>[3x]MSASPPISAGDYLSAPEPDALKPAGPTPSQSRFQVDLVTESAGDGETTVGFDSSPPEYVAEPPPDGLRDSVSGGEKAKGRFRVVNFAASSPDAAPAETAQNGDTVMSEGSLHSSTGGQQHHHYDTHTNTYYLRTFGHNTIDAVPKIDFYRQTAAPLGEKLIRPTLSELHDELDKEPFEDGFANGEELTPAEESAAKDVSESKEPVRFGWVKGVMIRCMLNIWGVILYLRLPWITAQAGIVLTWIIILLSVTVTSITGLSISAISTNGKVKSGGTYFLISRSLGPELGGSIGLIFAFANAVGVAMHTVGFAATVRDLLQEYGAPIVDPINDIRIIGVVSVTVLLAISLAGMEWESKAQVLFFLVIMVSFANYLVGTLIPPSEDKASKGFFSYRADIFVQNLVPDWRGPDGTFFGMFSIFFPSATGILAGANISGDLKDPAIAIPKGTLMAIFWTTISYLAISATIGSCVVRDASGVLNDTVTPGWGACEGLACSYGWNFTECTQQHSCHYGLINYYQTMSMVSGFAPLITAGIFGATLSSALACLVSAAKVFQCLCEDQLYPLIGF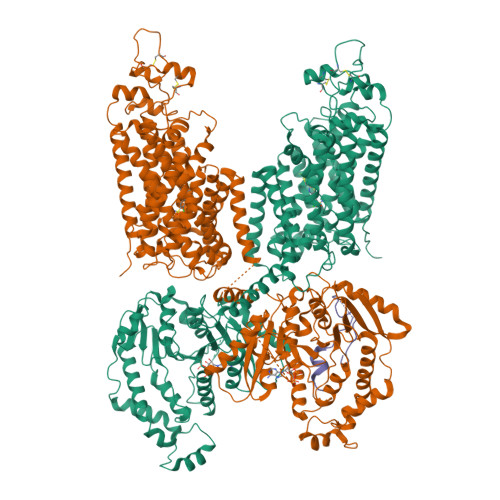FGKGYGKNKEPVRGYLLAYAIAVAFIIIAELNTIAPIISNFFLCSYALINFSCFHASITNSPGWRPSFQYYNKWAALFGAIISVVIMFLLTWWAALIAIGVVLFLLLYVIYKKPEVNWGSSVQAGSYNLALSYSVGLNEVEDHIKNYRPQCLVLTGPPNFRPALVDFVGTFTRNLSLMICGHVLIGPHKQRMPELQLIANGHTKWLNKRKIKAFYSDVIAEDLRRGVQILMQAAGLGRMKPNILVVGFKKNWQSAHPATVEDYIGILHDAFDFNYGVCVMRMREGLNVSKMMQAHINPVFDPAEDGKEASARVDPKALVKEEQATTIFQSEQGKKTIDIYWLFDDGGLTLLIPYLLGRKRRWSKCKIRVFVGGQINRMDQERKAIISLLSKFRLGFHEVHILPDINQNPRAEHTKRFEDMIAPFRLNDGFKDEATVNEMRRDCPWKISDEEITKNRVKSLRQVRLNEIVLDYSRDAALIVITLPIGRKGKCPSSLYMAWLETLSQDLRPPVILIRGNQENVLTFYCQ>[2x]MKLWFSTLKLKKAAAVLLFSCVA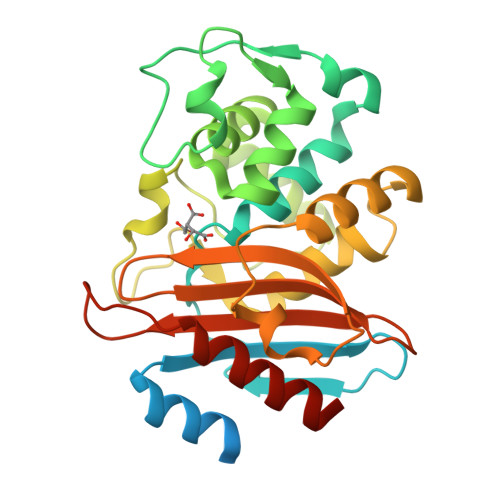LAGCANNQTNASQPAEKNEKTEMKDDFAKLEEQFDAKLGIFALDTGTNRTVTYRPDERFAFASTIKALTVGVLLQQKSIEDLNQRITYTRDDLVNYNPITEKHVDTGMTLKELADASLRYSDNTAQNLILKQIGGPESLKKELRKIGDEVTNPERFEPELNEVNPGETQDTSTARALATSLQAFALEDKLPSEKRELLIDWMKRNTTGDALIRAGVPEGWEVADKTGAGSYGTRNDIAIIWPPKGDPVVLAVLSSRDKKDAKYDDKLIAEATKVVVKALNMNGK Transcription initiation of snRNA genes relies on a specific factor called snRNA-activating protein complex (SNAPc). SNAPc binds a DNA motif in the upstream region of snRNA promoters, referred to as the proximal sequence element (PSE). The core of SNAPc binds two turns of DNA and recognizes the snRNA promoter-specific proximal sequence element (PSE), located upstream of the TATA box-binding protein TBP. Two extensions of SNAPc, called wing-1 and wing-2, bind TFIIA and TFIIB, respectively, explaining how SNAPc directs Pol II to snRNA promoters.

To obtain a high-resolution structure of SNAPc, we additionally reconstituted a SNAPc-containing Pol II PIC on DNA that was based on the U5 promoter sequence. The resulting cryo-EM dataset enabled refinement of the SNAPc-containing PIC in the CC state at an overall resolution of 3.0 Å and with the local map of the upstream region extending to 3.2 Å. The local map enabled building of an atomic model for SNAPc and PSE-containing upstream DNA. The high-resolution structure of the SNAPc-core bound to the U5 promoter shows how the subunits SNAPC1, SNAPC3 and SNAPC4 fold and interact. The SNAPc-core is stabilized by intricate interactions of SNAPC3 with both SNAPC1 and SNAPC4. SNAPc also contains two protrusions that we refer to as ‘wing-1’ and ‘wing-2. Whereas wing-1 of SNAPc binds to TFIIA, wing-2 binds TFIIB. SNAPc interaction with TFIIA and TFIIB involves three interfaces that we call A, B and C. In interface A, the wing-1 of SNAPC4 (helices α4 and α5) slides under the four-helix bundle of TFIIA like a wedge, stabilizing the flexible bundle region. Interface C is formed between wing-2 and the C-terminal cyclin fold of the TFIIB core. Although biochemical studies had identified SNAPC3 and SNAPC4 as poor DNA binders when investigated in isolation, our results suggest that formation of the SNAPc complex with its intricate interactions between these two subunits enables tight binding of the PSE, which explains how SNAPc recognizes the snRNA promoter.

> MASTSRLDALPRVTCPNHPDAILVEDYRAGDMICPECGLVVGDRVIDVGSEWRTFSNDKATKDPSRVGDSQNPLLSDGDLSTMIGKGTGAASFDEFGNSKYQNRRTMSSSDRAMMNAFKEITTMADRINLPRNIVDRTNNLFKQVYEQKSLKGRANDAIASACLYIACRQEGVPRTFKEICAVSRISKKEIGRCFKLILKALETSVDLITTGDFMSRFCSNLCLPKQVQMAATHIARKAVELDLVPGRSPISVAAAAIYMASQASAEKRTQKEIGDIAGVADVTIRQSYRLIYPRAPDLFPTDFKFDTPVDKLPQL;> MDQNNSLPPYAQGLASPQGAMTPGIPIFSPMMPYGTGLTPQPIQNTNSLSILEEQQRQQQQQQQQQQQQQQQQQQQQQQQQQQQQQQQQQQQQQQAVAAAAVQQSTSQQATQGTSGQAPQLFHSQTLTTAPLPGTTPLYPSPMTPMTPITPATPASESSGIVPQLQNIVSTVNLGCKLDLKTIALRARNAEYNPKRFAAVIMRIREPRTTALIFSSGKMVCTGAKSEEQSRLAARKYARVVQKLGFPAKFLDFKIQNMVGSCDVKFPIRLEGLVLTHQQFSSYEPELFPGLIYRMIKPRIVLLIFVSGKVVLTGAKVRAEIYEAFENIYPILKGFRKTT;> MANSANTNTVPKLYRSVIEDVINDVRDIFLDDGVDEQVLMELKTLWENKLMQSRAVDGFHSEEQQLLLQVQQQHQPQQQQHHHHHHHQQAQPQQTVPQQAQTQQVLIPASQQATAPQVIVPDSKLIQHMNASNMSAAATAATLALPAGVTPVQQILTNSGQLLQVVRAANGAQYIFQPQQSVVLQQQVIPQMQPGGVQAPVIQQVLAPLPGGISPQTGVIIQPQQILFTGNKTQVIPTTVAAPTPAQAQITATGQQQPQAQPAQTQAPLVLQVDGTGDTSSEEDEDEEEDYDDDEEEDKEKDGAEDGQVEEEPLNSEDDVSDEEGQELFDTENVVVCQYDKIHRSKNKWKFHLKDGIMNLNGRDYIFSKAIGDAEW;> MAYQLYRNTTLGNSLQESLDELIQSQQITPQLALQVLLQFDKAINAALAQRVRNRVNFRGSLNTYRFCDNVWTFVLNDVEFREVTELIKVDKVKIVACDGKNTGSNTTE;> MGTPPGLQTDCEALLSRFQETDSVRFEDFTELWRNMKFGTIFCGRMRNLEKNMFTKEALALAWRYFLPPYTFQIRVGALYLLYGLYNTQLCQPKQKIRVALKDWDEVLKFQQDLVNAQHFDAAYIFRKLRLDRAFHFTAMPKLLSYRMKKKIHRAEVTEEFKDPSDRVMKLITSDVLEEMLNVHDHYQNMKHVISVDKSKPDKALSLIKDDFFDNIKNIVLEHQQWHKDRKNPSLKSKTNDGEEKMEGNSQETERCERAESLAKIKSKAFSVVIQASKSRRHRQVKLDSSDSDSASGQGQVKATRKKEKKERLKPAGRKMSLRNKGNVQNIHKEDKPLSLSMPVITEEEENESLSGTEFTASKKRRKH;> MAEGSRGGPTCSGVGGRQDPVSGSGGCNFPEYELPELNTRAFHVGAFGELWRGRLRGAGDLSLREPPASALPGSQAADSDREDAAVARDLDCSLEAAAELRAVCGLDKLKCLEDGEDPEVIPENTDLVTLGVRKRFLEHREETITIDRACRQETFVYEMESHAIGKKPENSADMIEEGELILSVNILYPVIFHKHKEHKPYQTMLVLGSQKLTQLRDSIRCVSDLQIGGEFSNTPDQAPEHISKDLYKSAFFYFEGTFYNDKRYPECRDLSRTIIEWSESHDRGYGKFQTARMEDFTFNDLCIKLGFPYLYCHQGDCEHVIVITDIRLVHHDDCLDRTLYPLLIKKHWLWTRKCFVCKMYTARWVTNNDSFAPEDPCFFCDVCFRMLHYDSEGNKLGEFLAYPYVDPGTFN;> MDVDAEREKITQEIKELERILDPGSSGSHVEISESSLESDSEADSLPSEDLDPADPPISEEERWGEASNDEDDPKDKTLPEDPETCLQLNMVYQEVIQEKLAEANLLLAQNREQQEELMRDLAGSKGTKVKDGKSLPPSTYMGHFMKPYFKDKVTGVGPPANEDTREKAAQGIKAFEELLVTKWKNWEKALLRKSVVSDRLQRLLQPKLLKLEYLHQKQSKVSSELERQALEKQGREAEKEIQDINQLPEEALLGNRLDSHDWEKISNINFEGSRSAEEIRKFWQNSEHPSINKQEWSREEEERLQAIAAAHGHLEWQKIAEELGTSRSAFQCLQKFQQHNKALKRKEWTEEEDRMLTQLVQEMRVGSHIPYRRIVYYMEGRDSMQLIYRWTKSLDPGLKKGYWAPEEDAKLLQAVAKYGEQDWFKIREEVPGRSDAQCRDRYLRRLHFSLKKGRWNLKEEEQLIELIEKYGVGHWAKIASELPHRSGSQCLSKWKIMMGKKQGLRRRRRRARHSVRWSSTSSSGSSSGSSGGSSSSSSSSSEEDEPEQAQAGEGDRALLSPQYMVPDMDLWVPARQSTSQPWRGGAGAWLGGPAASLSPPKGSSASQGGSKEASTTAAAPGEETSPVQVPARAHGPVPRSAQASHSADTRPAGAEKQALEGGRRLLTVPVETVLRVLRANTAARSCTQKEQLRQPPLPTSSPGVSSGDSVARSHVQWLRHRATQSGQRRWRHALHRRLLNRRLLLAVTPWVGDVVVPCTQASQRPAVVQTQADGLREQLQQARLASTPVFTLFTQLFHIDTAGCLEVVRERKALPPRLPQAGARDPPVHLLQASSSAQSTPGHLFPNVPAQEASKSASHKGSRRLASSRVERTLPQASLLASTGPRPKPKTVSELLQEKRLQEARAREATRGPVVLPSQLLVSSSVILQPPLPHTPHGRPAPGPTVLNVPLSGPGAPAAAKPGTSGSWQEAGTSAKDKRLSTMQALPLAPVFSEAEGTAPAASQAPALGPGQISVSCPESGLGQSQAPAASRKQGLPEAPPFLPAAPSPTPLPVQPLSLTHIGGPHVATSVPLPVTWVLTAQGLLPVPVPAVVSLPRPAGTPGPAGLLATLLPPLTETRAAQGPRAPALSSSWQPPANMNREPEPSCRTDTPAPPTHALSQSPAEADGSVAFVPGEAQVAREIPEPRTSSHADPPEAEPPWSGRLPAFGGVIPATEPRGTPGSPSGTQEPRGPLGLEKLPLRQPGPEKGALDLEKPPLPQPGPEKGALDLGLLSQEGEAATQQWLGGQRGVRVPLLGSRLPYQPPALCSLRALSGLLLHKKALEHKATSLVVGGEAERPAGALQASLGLVRGQLQDNPAYLLLRARFLAAFTLPALLATLAPQGVRTTLSVPSRVGSESEDEDLLSELELADRDGQPGCTTATCPIQGAPDSGKCSASSCLDTSNDPDDLDVLRTRHARHTRKRRRLV;> MLSRLQELRKEEETLLRLKAALHDQLNRLKVEELALQSMISSRRGDEMLSSHTVPEQSHDMLVHVDNEASINQTTLELSTKSHVTEEEEEEEEEESDS N-[(4-methylpyrimidin-2-yl)carbamoyl]-2-nitrobenzenesulfonamide | C12 H11 N5 O5 S | 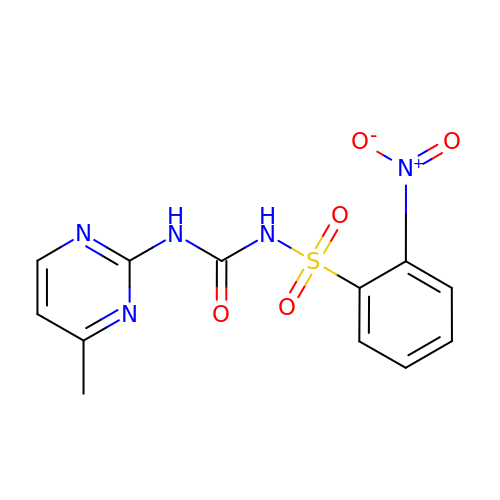DPIRXVCCFDCYGI-UHFFFAOYSA-N>MGSSHHHHHHSQDPANRNVPIPRRQLYIGGEWREPVKKNRIPIINPATEEIIGDIPAATAEDVDIAVEAARKAIARDDWGSTTGAQRAKYLRAIAAKVLEKKSVLATLESLDSGKTLYESAADMDDVAGCFEYYAGLAEALDSRRMTPVNLNSDSYKSYVLREPLGVVGLITPWNYPLLMAIWKVAPALAAGCAAILKPSELASITCLELGEICREIGLPSGALNILTGLGPEAGGPLASHPHVDKISFTGSGPTGSKIMTAAAQLVKPVSLELGGKSPIVVFDDIDNLDIAAEWTLFGIFANTGQVCSATSRLIVQENIASAFMDRLLKWTKNIKISDPLEEDCKLGPVVSAGQYEKVLKFISN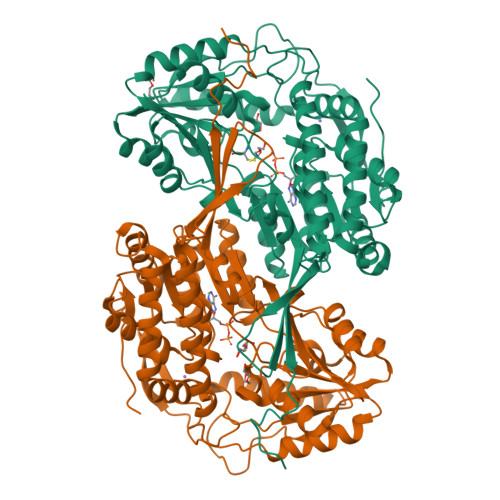AKSEGATILCGGERPQHLKKGYYVQPTIITDVNTSMEIWKEEVFGPVLCVKTFKTEEQAIELANDTKYGLGAAVMSKDVKRCERFTKAFQTGIIWINCSQPTFNELPWGGKKRSGFGRDLGKWGLENFLNIKQVTEYTSAEPLAFYKSPSKN[2x]(2R)-2-[(2S,3R)-1,3-bis(oxidanyl)-1-oxidanylidene-butan-2-yl]-4-(2-methanimidamidoethylsulfanyl)-2,3-dihydro-1H-pyrrole-5-carboxylic 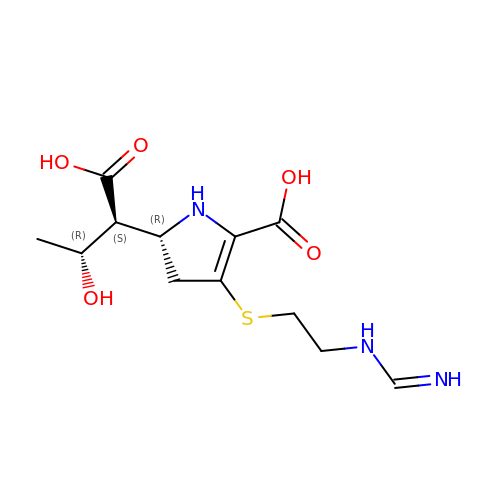acid | C12 H19 N3 O5 S | KSLAOLVLEKIZMQ-ZXFLCMHBSA-N N-[(4-methoxyphenyl)methyl]quinoxaline-6-carboxamide 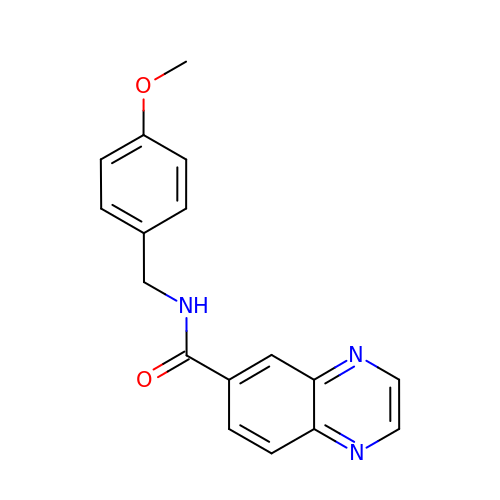| C17 H15 N3 O2 | CQHKQYSHFWCLKE-UHFFFAOYSA-N>[4x]MQPHLFTPLTIGSVTLRNRIGMSPMCQYSAVDGFPTDWHLMHLGARAAGGVGLIILEATAVSPEGRISPFDLGIWSDDHIAALSRIVKLIESLGAVAGIQLAHAGRKASVGRPWEGGKPIAPANGGWPVVGPT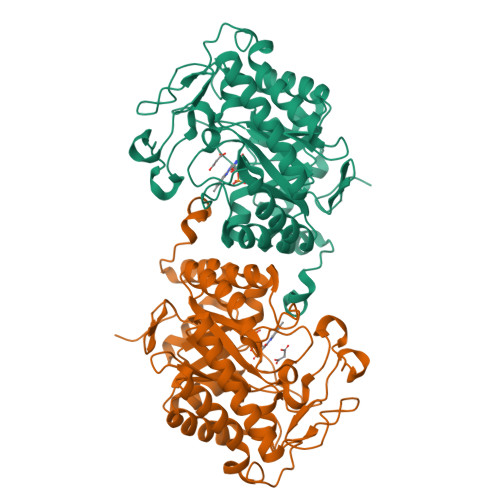AEPFAPGYPTPIPLDAAGIARVVADFATATKRARAAGFRWIEIHAAHGYLLHNFLSPLGNDRNDEYGGDLRGRVRLLSEVTAAVRAEWPSDLPLAVRLSCSDWTPEGLTIADTVEVARMLREQGVDLIDCSSGGIAPGITIPVGEGYQVPFAAQVRREANIATAAVGLITRPEHADAIVRNGDADLVLLGRELLRDPHWPLRAARALGHDLAPPPQYLRAW> GVVEHCCHRPCSNAEFKKYC;> TFDTPKHRCGSEITNSYMDLC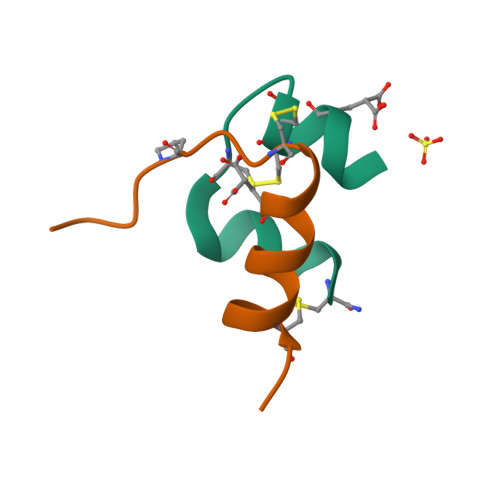YR>[4x]GAVDADSANYRIEHDTMGEVRVPAKALWRAQTQRAVENFPISGRGLERTQIRALGLLKGACAQVNSDLGLLAPEKADAIIAAAAEIADGQHDDQFPIDVFQTGSGTSSNMNTNEVIASIAAKGGVTLHPNDDVNMSQSSNDTFPTATHIAATEAAVAHLIPALQQLHDALAAKALDWHTVVKSGRTHLMDAVPVTLGQEFSGYARQIEAGIERVRACLPRLGELAIGGTAVGTGLNA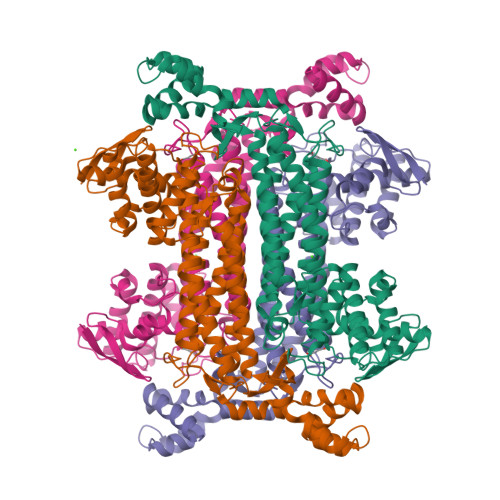PDDFGVRVVAVLVAQTGLSELRTAANSFEAQAARDGLVEASGALRTIAVSLTKIANDIRWMGSGPLTGLAEIQLPDLQPGCSIMPGKVNPVLPEAVTQVAAQVIGNDAAIAWGGANGAFELNVYIPMMARNILESFKLLTNVSRLFAQRCIAGLTANVEHLRRLAESSPSIVTPLNSAIGYEEAAAVAKQALKERKTIRQTVIDRGLIGDRLSIEDLDRRLDVLAMAKAEQLDSDRL> SRKKMGLLVMAYGTPYKEEDIERYYTHIRRGRKPEPEMLQDLKDRYEAIGGISPLAQITEQQAHNLEQHLNEIQDEITFKAYIGLKHIEPFIEDAVAEMHKDGITEAVSIVLAPHFSTFSVQSYNKRAKEEAEKLGGLTITSVES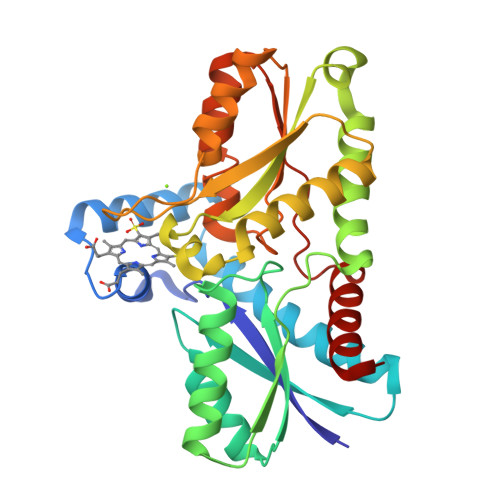WYDEPKFVTYWVDRVKETYASMPEDERENAMLIVSACSLPEKIKEFGDPYPDQLHESAKLIAEGAGVSEYAVGWQSEGNTPDPWLGPDVQDLTRDLFEQKGYQAFVYVPVGFVADHLEVLYDNDYECKVVTDDIGASYYRPEMPNAKPEFIDALATVVLKKLGR>[8x]MQIRDWLPLLGMPLMLLFVQIIAIVLVMPMQAAGLVAFENPSSVANPLIFIGMLLAFTLVLLVLLRTGGRRFIAAFIGFALFMT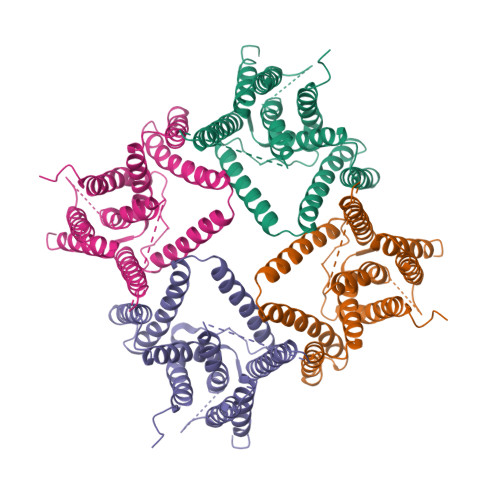FLYIFGALSLLALGPTTAAAAGTLIGAVAVTALLYLYPEWYVIDILGVLISAGVASIFGISLEPLPVLVLLVLLAVYDAISVYRTKHMITLAEGVLETKAPIMVVVPKRADYSFRKEGLNISEGEERGAFVMGMGDLIMPSILVVSSHVFVDAPAVLWTLSAPTLGAMVGSLVGLAVLLYFVNKGNPQAGLPPLNGGAILGFLVGAALAGSFSWLPF(2E)-2-{[(Z)-{3-HYDROXY-2-METHYL-5-[(PHOSPHONOOXY)METHYL]PYRIDIN-4(1H)-YLIDENE}METHYL]IMINO}-4-(METHYLSULFANYL)BUTANOIC ACID | C13 H19 N2 O7 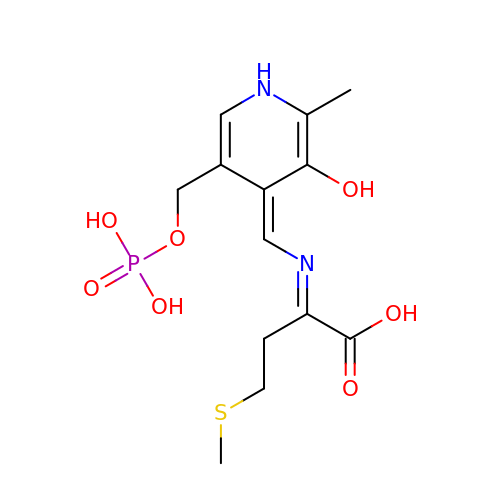P S | UNHRYMFMFMQCNK-JNVWRRHBSA-N Glyoxylate is a small and very reactive dicarboxylic acid molecule synthesized by most eukaryotes and prokaryotes. Considered as a toxic intermediate, this compound is metabolized by an unusual enzyme assigned to the D-2-hydroxy-acid dehydrogenase superfamily, glyoxylate reductase/hydroxypyruvate reductase (GRHPR). First, GRHPR is a dual activity enzyme. It catalyzes the reduction of glyoxylate into glycolate, which is either excreted or reconverted into glyoxylate (futile cycle) and the conversion of hydroxypyruvate into D-glycerate, a precursor supplying in the gluconeogenic pathway carbon.

To go deeper in the specificity of these enzymes, we determined the crystal structures of PfuGRHPR and PyaGRHPR at 1.4 Å and 2.0 Å resolution, respectively. The asymmetric unit of PyaGRHPR crystal displays a full dimer. The electron density maps obtained revealed that Pfu and PyaGRHPR enzymes are in ternary (enzyme + cofactor + substrate/product) form. Neither cofactors nor substrates were added during the crystallization or the cryoprotection step. Both structures include a cofactor molecule, unambiguously modeled as NADP(H), within each active site with a refined occupancy of 100%. The PyaGRHPR structure contains D-glycerate, product of HPR activity as observed in the holo form of human GRHPR12. Contrary to what was observed in hGRHPR structure, both active sites in the PyaGRHPR dimer are occupied with a D-glycerate molecule. The conserved Arg241 was proposed to orient and to hold the substrate for catalysis through two hydrogen bonds with the 2-hydroxyl and carboxyl groups of D-glycerate respectively. Additional interactions for substrate orientation are provided through carboxylate oxygen atoms forming charged hydrogen bonds with the main chain amines of Val76 and Gly77. In the PyaGRHPR structure in the presence of D-glycerate, the network Trp138, Ser291 and Arg297 superposes strictly with the one identified in the human structure12.

>[2x]MKPKVLITRAIPENGIELLREHFEVEVWEHEHEIPREVLLEKVKDVDALVTMLSEKIDREVFDAAPRLRIVANYAVGYDNIDIEEATKRGIYVTNTPDVLTDATADLAWALLLAAARHVVKGDKFVRSGEWKRRGIAWHPKMFLGYDVYGKTIGIVGFGRIGQAIAKRAKGFGMRILYTARSRKPEAEKELGAEFKPLEELLRESDFVVLAVPLTKETYHMINEERLRLMKPTAVLVNVARGKVVDTKALIRALKEGWIAAAGLDVFEEEPYYDEELFALDNVVLTPHIGSATFGAREGMAELVAKNLIAFKNGEVPPTLVNREVLKVRRPGF(2R)-2-(phosphonooxy)propanoic acid | C3 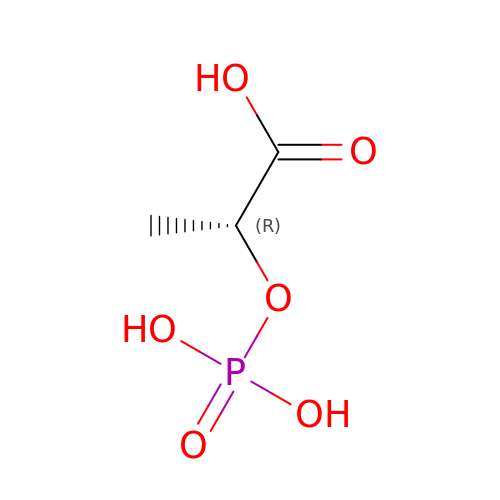H7 O6 P | CSZRNWHGZPKNKY-UWTATZPHSA-N> ANGSVCNTCPEAWIYFQKKCYYFGEGAKKWIQARYACENLHGRLVSIHSPEEQDFLTKRANW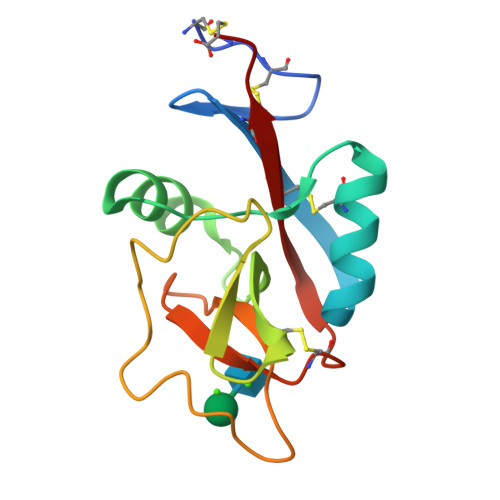RGSWIGLRDLDIEGEFIWMDNQPLDYSNWQPGEPNDAGQGENCVMMLGSGKWNDAFCGSELHGWVCDRLATC> GSMGVFTCTLADITSPVAPARLFQAFTIDNHNLMPKVVPQFVKSIDFVQGDSTAVGCVKQINFPADAPFTYVKNRVDEIDASKYYLKYTCIEGDAFPDTVEYAVYEDTFEQTETGSRCKMVAHYHLKGDSVMKEEDVAPAKEGIQKMFKAVEEHLIANPQLYA

Here, we isolated a salt-induced PR-10 gene from the halophyte Halostachys caspica and named it HcPR10. Like the structures of other PR-10 proteins (Aglas et al., 2020; Morris et al., 2021), HcPR10 was composed of a seven-stranded β-sheet (β1-β7), two closely connected V-shaped α-helices (α1-α2) between β1 and β2, a long C-terminal α-helix (α3) and eight loops (L1-L8) connecting these structural elements. HcPR10 formed a pinecone-shaped structure, with the twisted seven-stranded β-sheet and the long C-terminal helix forming the top surface of this structure and the curved V-shaped helices forming the bottom. The structural analysis support that HcPR10 is a cytokinin-binding protein that acts as a reservoir for cytokinins and helps maintain cytokinin homeostasis, thereby guaranteeing stable transmission of cytokinin signals in plant cells.

Inside the pinecone-shaped structure was a large cavity mainly composed of hydrophobic residues that may favor hydrophobic ligand binding. The cavity also contained several hydrophilic residues, allowing water molecules to bind inside the cavity in the apo-form structure. The cavity had a volume of ~1,339 Å3 and contained one entrance located at the surface close to the top of the pinecone-shaped structure. The entrance was surrounded by the long C-terminal helix, loops connecting α2, and β2 (L2), β3 and β4 (L4) and β5 and β6 (L6). The entrance was approximately 5.9 Å wide and 16 Å long, which was large enough for the internal insertion of a small ligand. We determined that recombinant HcPR10 took on the structure of a typical PR-10 protein, with a pinecone-like shape and a large hydrophobic cavity in the middle.>[2x]GKDGSNSLAEIRTDFNILYSMMKKHEEFRWMRLRIRRMADAWIQAIKSLAEKQNLEKRKRKKVLVHLGLLTKESGFKIAETAFSGGPLGELVQWSDLITSLYLLGHDIRISASLAELKEIMKGGGGIVELIYIDIVGLAQFKKTLGPSWVHYQCMLRVLDSFGTEPEFNHANYAQSKGHKTPWGKWNLNPQQFYTMFPHTPDNSFLGFVVEQHLNSSDIHHINEIKRQNQSLVYGKVDSFWKNKKIYLDIIHTYMEVHATVYGSSTKNIPSYVKNHGILSGRDLQFLLRETKLFVGLGFPYEGPAPLEAIANGCAFLNPKFNPPKSSKNTDFFIGKPTLRELTSQHPYAEVFIGRPHVWTVDLNNQEEVEDAVKAILNQKIEPYMPYEFTCEGMLQRINAFIEKQDFCHGQVMWPPLSALQVKLAEPGQSCKQVCQESQLICEPSFFQHLNKDKDMLKYKVTCQSSELAKDILVPSFDPKNKHCVFQGDLLLFSCAGAHPRHQRVCPCRDFIKGQVALCKDCL

Human GnT-V is a type II membrane protein and comprises 741 amino acids in total. GnT-V acts only on the α1-6 mannose branch of N-glycans, and this process is highly regulated. Mechanistically, the β1-6 branch glycan modification by GnT-V allows target proteins to be decorated with a number of N-acetyllactosamine (LacNAc) residues, creating high-affinity ligands for galectins. In this study, we determined the crystal structures of the GnT-V catalytic domain in an apo form and in complex with our bisubstrate-type inhibitor as a substrate analog.

Consequently, we designed a new truncated construct of GnT-V luminal domain, mini-GnT-V, in which N-terminal domain (T121-N212) was deleted. Also, the long unstructured loop (K330-R344), involved in an interregional disulfide bond (C172-C338), was replaced with a short linker of four glycine residues to reduce the structural heterogeneity. We further introduced the inactive E297A mutation to mini-GnT-V to form a stable complex with ligand. Crystal structure of mini-GnT-V E297A mutant in complex with the ligand was successfully determined at 2.1 Å resolution. The asymmetric unit contains two mini-GnT-V inhibitor complexes, referred to as complex A and B. Structural superposition of the two complexes demonstrated that overall RMSD value of Cα atoms is only 0.76 Å. Of note, one difference is that the weak electron density of a highly mobile region (G282-G296) is observed in complex B and included in the final model. The trisaccharide moiety binds to mini-GnT-V between the two middle domains. Among the three sugar residues, both GlcNAc-3 and Man-2 are buried in the cavity and tightly bind to mini-GnT-V via direct and water-mediated interactions, whereas Man-1 is exposed to solvent. Notably, two aromatic rings of F380 and W401 contact the trisaccharide and the side chain of W401 and seem to restrain the conformation of the α1-6 branch. We applied the bisubstrate inhibitor for co-crystallization, but the electron density of the donor moiety was completely missing.> GPLGSMDEDVLPGEVLAIEGIFMACGLNEPEYLYHPLLSPIKLYITGLMRDKESLFEAMLANVRFHSTTGINQLGLSMLQVSGDGNMNWGRALAILTFGSFVAQKLSNEPHLRDFALAVLPAYAYEAIGPQWFRARGGWRGLKAYCTQVLT;> SESQEDIIRNIARHLAQVGDSMDRSIPPGLVNGL

Kaposi sarcoma herpes virus (KSHV), a member of the gammaherpesvirinae, has been shown to encode for KsBcl-2, a potent inhibitor of Bcl-2 mediated apoptosis. KsBcl-2 acts by directly engaging host pro-apoptotic Bcl-2 proteins including Bak, Bax and Bok, the BH3-only proteins; Bim, Bid, Bik, Hrk, Noxa and Puma. We also show KsBcl-2 adopts a globular conserved monomeric Bcl-2-fold structure similar to other characterized herpes virus encoded Bcl-2 homologs and binds BH3 motif peptides using the canonical Bcl-2 ligand binding groove. KsBcl-2 lacks any significant shared sequence identity with mammalian Bcl-2 proteins though it does contain a recognizable “NWGR” sequence motif in the BH1 region, which is crucial for pro-survival function of majority of Bcl-2 family proteins.

The KsBcl-2:Bid complex was refined to 1.41 Å, whereas the KsBcl-2:Puma complex was refined to 2.11 Å. Clear and continuous electron density was observed for KsBcl-2 residues 1–146 and Bid residues 79–104 in the KsBcl-2: Bid BH3 complex, as well as KsBcl-2 residues 1–146 and Puma residues 130–155 in the KsBcl-2: Puma BH3 complex. The crystal structure of a KsBcl-2: Bid BH3 complex revealed that as previously seen for the related BHRF-1 and cellular Mcl-1, KsBcl-2 adopts a typical Bcl-2 fold with globular monomeric topology with eight alpha-helices and alpha-helices 2–5 form the canonical hydrophobic ligand binding groove. Binding of Bid BH3 peptide to KsBcl-2 occurs via the canonical ligand binding groove that is formed by helices α2–α5. The four canonical BH3 motif defining residues from Bid, I89, L93 and V96 and M100, are bound in four hydrophobic pockets of the ligand binding groove. A fifth hydrophobic pocket in KsBcl-2 is occupied by Bid I85. The hallmark ionic interaction between pro-survival Bcl-2 proteins and pro-apoptotic BH3 motif ligands between a conserved arginine (R86KsBcl-2) in the BH1 motif and aspartate (D98BID) of the Bid BH3-motif is also present. This interaction is supplemented by multiple hydrogen bonding interactions between Q82BID and Q68KsBcl-2, I86BID and S72KsBcl-2, D98BID and N83KsBcl-2, D101BID and G85KsBcl-2, R102BID and Y140KsBcl-2 as well as between R102BID and T146KsBcl-2. A comparison of overall fold of the KsBcl-2: Bid BH3 complex reveals that it is very similar to that observed in other Bcl-2: BH3 complexes. For the KsBcl-2:Bid complex this additional hydrophobic pocket is utilized by N-terminal residue I85BID and in KsBcl-2:Puma complex this additional hydrophobic pocket is utilized by W133PUMA.Patched 1, GPR161, SMO and other ciliary membrane proteins are all ferried out of cilia in a regulated manner by an evolutionarily conserved complex of eight Bardet-Biedl Syndrome (BBS) proteins, the BBSome. Our recent cryo-electron microscopy (cryo-EM) structure of the BBSome revealed that the BBSome exists mostly in an auto-inhibited, closed conformation in solution and undergoes a conformational change as it is recruited to membranes by ARL6GTP. Given that ARL6GTP triggers polymerization of a membrane-apposed BBSome/ARL6 coat and enables BBSome-mediated TZ crossing, the ARL6GTP-bound BBSome conformation represents the active form of the complex. Here we determine high-resolution structures of the BBSome alone and bound to ARL6GTP, and we map the BBSome–SMO interaction to model how the membrane-associated BBSome–ARL6GTP complex recognizes its cargoes.

Mixing recombinant ARL6GTP together with the purified BBSome allowed for complex formation in solution. The BBSome–ARL6GTP complex was analyzed by cryo-EM, yielding a density map at an overall resolution of 4.0 Å. Focused refinement of the top and lower lobes of the complex resulted in improved maps of 3.8 Å and 4.2 Å resolution, which facilitated model building. In the BBSome–ARL6 structure, ARL6GTP is nestled in a wedge opening between BBS1βprop and BBS7βprop. A ~ 20° rotation of BBS1βprop from the BBSome alone conformation allows ARL6GTP to move away from the steric clash with BBS2βprop. This movement of BBS1βprop is accompanied by a twisting of the first two TPR repeats from the BBS4 α-solenoid, in line with the close association between the N terminus of BBS4 and BBS1βprop seen in the BBSome alone structure and confirmed by cross-link mass spectrometry. Besides the movements of BBS1βprop and BBS4TPR1-2, ARL6GTP binding caused only subtle changes in the structure of the BBSome. As previously found in the crystal structure of the BBS1βprop–ARL6GTP complex, the BBS1βprop makes contacts with the Switch 2 region and with helix α3 of ARL6GTP while the Switch 1 region of ARL6 is readily available for interacting with other, yet unidentified, complexes. Interestingly, the ‘backside’ of ARL6GTP (i.e., the surface on the opposite side of the Switch regions) interacts with a loop that connects BBS7βprop and BBS7cc. In addition, the physical interaction between ARL6GTP and the upper lobe removes the upper lobe flexibility previously observed in the BBSome alone preparation, resulting in a more stable BBSome conformation.

> MGLLDRLSGLLGLKKKEVHVLCLGLDNSGKTTIINKLKPSNAQSQDIVPTIGFSIQKFKSSSLSFTVFDMSGQGRYRNLWEHYYKEGQAIIFVIDSSDKLRMVVAKEELRTLLNHPDIKHRRIPILFFANKMDLRDALTSVKVSQLLCLEDIKDKPWHICASDAIKGEGLQEGVDWLQDQIQSVKT;> MLQPVFTLKLRHKISPRMVAVGRYDGTHPCLAAATQAGKVFIHNPHSRSQHLGAPRVLQSPLESDVSLLNINQTVSCLTAGVLNPELGYDALLVGTQTNLLAYDVYNNSDLFYREVADGASAIVLGTLGDITSPLAIIGGNCALQGFNHEGNDLFWTVTGDNVHSLALCDFDGDGKKELLVGSEDFDIRVFKEDEIVAEMSETEIITSLCPMYGSRFGYALSNGTVGVYDKTARYWRIKSKNQAMSIHAFDLNSDGVCELITGWSNGKVDARSDRTGEVIFKDNFSSAIAGVVEGDYRMEGCQQLICCSVDGEIRGYLPGTAEMRGNLMDISVEQDLIRELSQKKQNLLLELRNYEENAKAELSSPLNEADGHRGVIPANTKHHTALSVSLGSEAQAAHAELCISTSNDTIIRAVLIFAEGVFAGESHVVHPSVHHLSSSVRIPITPPKDIPVDLHLKTFVGYRSSTQFHVFELTRQLPRFSMYALTSPDPASEPLSYVNFIIAERAQRVVMWLNQNFLLPEDTNIQNAPFQVCFTSLRNGGQLYIKIKLSGEITVNTDDIDLAGDIIQSMASFFAIEDLQVEADFPVYFEELRKVLVKVDEYHSVHQKLSADMADNSNLIRSLLVQAEDARLMRDMKTMKNRYKELYDLNKDLLNGYKIRCNNHTELLGSLKAVNQAIQRAGHLRVGKPKNQVITACRDAIRSNNINMLFRIMRVGTASS;> MDLNLNRADYLQVGVTSQKTMKLLPASKHRATQKVVVGDHDGIVMCFGMKKGEAVTVFKTLPGQKIARLELGGALNTPQEKIFIAAGSEIRGFTKRGKQFLSFETNLTESIKAMHISGSDLFLSASYIYNHYCDCKDQHYYLSGDKINDVICLPVERLLREVPVLACQDRVLRVLQGSDVTYEIEVPGPPTVLALHNGNGGDSGEDLLFGTSDGKLGLIQITTSKPIHKWEIRNEKKRGGILCVDSFDIVGDGVKDLLVGRDDGMVEVYGFDNANEPVLRFDHTLSESVTSIQGGCVGKDGYDEIVVSTYSGWITGLTTEPVHKESGPGEELKFNQEMQNKISSLRSELEQLQYKVLQEREKYQQSSQSSKAKSAVPSFSVNDKFTLNKDDASYSLILEVQTAIDNVLIQSDVPIDLLDVDKNSAVVSFSSCDSESNDNFLLATYRCQANTTRLELKIRSIEGQYGTLQAYVTPRIQPKTCQVRQYHIKPLSLHQRTHFIDHDRPMNTLTLTGQFSFSELHSWVVFCMPEVPEKPPAGECVTFYFQNTFLDTQLESTYRKGEGVFKSDNISTISILKDVLSKEATKRKINLNISYEINEVSVKHTLKLIHPKLEYQLLLAKKVQLIDALKELQVHEGNTNFLIPEYRCILEEADHLQEEYKKQPAHLERLYGMITDLFIDKFKFKGTNVKTKVPLLLEILDSYDQNALIAFFDAA;> MAATSSSDSDGGKGESEANSKWLDSLSDSMANIHTFSACLALADFHGDGEYKLAMGDLGPDGRQPRLKVLKGHTLVSQKPLPDLPAAAVTFLMASHEPRTPALAIASGPCVYVYKNLKPYFKFSLPSLPTNPLEQDLWNQAKEDQIDPLTLKEMLEGIREKAEVPLSVQSLRFLPLELSEMEAFVNQHKSKSIRRQTVITTMTTLKKNLADEDAVSCLVLGTENKELLVLDPEAFTILAKMSLPSVPAFLEASGQFDVEFRLAAACRNGSIYILRRDSKRPKYCIELGAQPVGLVGVHKVLVVGSNQDSLHGFTYKGKRLWTVQMPAAILAMNLLEQHSRGLQAVMAALANEEVRIYHDKVLLNVIRTPEAVTSLCFGRYGREDNTLIMTTLGGGLIIKILKRTAVFAEGGGEAGPPPSQAIKLNVPRKTRLYVDQTLREREAGTAMHRTFQADLYLLRLRAARAYVQALESSLSPVSLTAREPLKLHAVVQGLGPTFKLTLHLQNTSTARPILGLVVCFLYNEVLYALPRAFFKVPLLVPGLNYPLETFVKSLSDKGISDIIKVLVLREGQSTPLLSAHINMPMSEGLAAD;> MAEEKLSARTQLPVSAESQKPVLKKAPEFPILEKQNWLIHLYYIQKDYEACKAVIKEQLQETHGLCEYAIYVQALIFRLEGNIQESLRLFQMCAFLSPQCADNLKQVARSLFLLGKHKAAIEVYNEAAKLNQKDWEICHNLGVCYIYLKQFDKAQDQLHNALHLNRHDLTYIMLGKIFLLKGDLDKAIEIYKKAVEFSPENTELLTTLGLLYLQLGIYQKAFEHLGNTLTYDPTNYKAILAAGSMMQTHGDFDVALTKYKVVACAVIESPPLWNNIGMCFFGKKKYVAAISCLKRANYLAPLDWKILYNLGLVHLTMQQYASAFHFLSAAINFQPKMGELYMLLAVALTNLEDSENAKRAYEEAVRLDKCNPLVNLNYAVLLYNQGEKRDALAQYQEMEKKVNLLKYSSSLEFDPEMVEVAQKLGAALQVGEALVWTKPVKDPKSKHQTASTSKAAGFQQPLGSNQALGQAMSSAATCRKLSSGAGGTSQLTKPPSLPLEPEPTVEAQPTEASAQTREK;> MEPLLLAWSYFRRRRFQLCADLCTQMLEKSPCDQAAWILKARALTEMVYVDEIDVDEEGIAEMILDENAIAQVPRPGTSLKLPGTNQTGGPSPAVRPVTQAGRPITGFLRPSTQSGRPGTIEQAIKTPRTAYTARPIASSSGRFVRLGTASMLTSPDGPFINLSRLNLAKYAQKPKLAKALFEYIFHHENDVKTALDLAALSTEHSQYKDWWWKVQIGKCYYRLGLYREAEKQFKSALKQQEMVDTFLYLAKVYISLDQPLTALNLFKQGLDKFPGEVTLLCGIARIYEEMNNISSATEYYKEVLKQDNTHVEAIACIGSNHFYTDQPEVALRFYRRLLQMGVYNCQLFNNLGLCCFYAQQYDMTLTSFERALSLAENEEEVADVWYNLGHVAVGTGDTNLAHQCFRLALVSNNQHAEAYNNLAVLEMRRGHVEQAKALLQTASSLAPHMYEPHFNFATISDKIGDLQRSYAAAKKSEAAFPDHVDTQHLIKQLEQHFAML;> MSVLDALWEDRDVRFDVSSQQMKTRPGEVLIDCLDSVEDTKGNNGDRGRLLVTNLRIVWHSLALPRVNLSIGYNCILNITTRTANSKLRGQTEALYVLTKCNSTRFEFIFTNLVPGSPRLYTSLIAVHRAYETSKMYRDFKLRSALIQNKQLRLLPQENVYNKINGVWNLSSDQGNLGTFFITNVRIVWHANMNDSFNVSIPYLQIRSVKIRDSKFGLALVIESSQQSGGYVLGFKIDPVEKLQESVKEINSLHKVYSANPIFGVDYEMEEKPQPLEALTVKQIQDDVEIDSDDHTDAFVAYFADGNKQQDREPVFSEELGLAIEKLKDGFTLQGLWEVMN;> MAETKSMFREVLPKQGQLYVEDITTMVLCKPKLLPLKSLTLEKLEKMQQAAQDTIHQQEMTEKEQKITH;> MSLFKARDWWSTVLGDKEEFDQGCLCLADVDNTGNGQDKIIVGSFMGYLRIFNPHPVKTGDGAQAEDLLLEVHLRDPILQVEVGKFVSGTEMLHLAVLHSRKLCVYSVSGTLGNVEHGNQYQIKLMYEHNLQRTACNMTYGSFGGVKGRDLICIQSVDGMLMVFEQESYAFGRFLPGSLLPGPLAYSSRTDSFITVSSCHQVESYKYQVLAFATDADKRQETEQQKHGSGKRLVVDWTLNIGEQAIDICIVSFIQSASSVFVLGERNFFCLKDNGQIQFMKKLDYSPSCFLPYCSVSEGTINTLIGNHNNMLHIYQDVTLKWATQLPHVPVAVRVGCLHDLKGVIVTLSDDGHLQCSYLGTDPSLFQAPKVESRELNYDELDMELKELQKVIKNVNKSQDVWPLTEREDDLKVSAMVSPNFDSVSQATDVEVGADLVPSVTVKVTLKNRVALQKIKLSIYVQPPLVLTGDQFTFEFMAPEMTRTVGFSVYLKGSYSPPELEGNAVVSYSRPTERNPDGIPRVSQCKFRLPLKLVCLPGQPSKTASHKLTIDTNKSPVSLLSLFPGFAKQSEDDQVNVMGFRFLGGSQVTLLASKTSQRYRIQSEQFEDLWLITNELIIRLQEYFEKQGIKDFTCSFSGSVPLEEYFELIDHHFELRINGEKLEELLSERAVQFRAIQRRLLTRFKDKTPAPLQHLDTLLDGTYKQVIALADAVEENQDNLFQSFTRLKSATHLVILLIGLWQKLSADQIAILEAAFLPLQQDTQELGWEETVDAALSHLLKTCLSKSSKEQALNLNSQLGIPKDTSQLKKHITLFCDRLAKGGRLCLSTDAAAPQTMVMPGGCATIPESDLEGRSIDQDSSELFTNHKHLMVETPVPEVSPLQGVTE NAL is a class I aldolase, and its biological role is to cleave Neu5Ac, however, at favorable conditions, the reverse aldol condensation reaction can be utilized in vitro to synthesize Neu5Ac from pyruvate and ManNAc. In this paper, we describe the recombinant production, biochemical characterization and structure determination of a N-acetylneuraminate lyase from the psychrophilic bacterium A. salmonicida (AsNAL). Despite having less than about 25% sequence identity to the homologous structures of EcNAL, HiNAL, SaNAL and PmNAL, AsNAL shares similarity in the overall fold, being a TIM barrel consisting of a barrel of 7 parallel strands (the eighth strand is distorted) surrounded by 11 helices. Although the sequence identity between AsNAL and the other NALs is low, residues involved in catalysis and substrate binding are well conserved.

A crystallization condition, composed of 25% PEG 1.5 K and 20% glycerol, produced diamond shaped crystals. The crystals diffracted up to 1.65 Å and belong to the orthorhombic space group I222 with cell parameters of 67 x 86 x 118 Å3. The whole amino acid sequence from residue 1 to 297 could be traced in the electron density maps. Three of the His residues from the tag were also visible in the electron density maps. Electron density clearly larger than water molecules was interpreted as glycerol and ethylene glycol originating from the crystallization conditions. There is one molecule in the asymmetric unit, but the crystallographic symmetry generates the functional tetrameric quaternary structure. The active sites are pointing inwards toward the center of a donut shaped tetramer. The corresponding residue in AsNAL is Asn168. This residue points towards the substrate and is positioned closer to the substrate than what is the case for Thr167 from EcNAL, or for an in silico mutation to threonine for AsNAL. Our structure of AsNAL shows that Asn168 is able to form two hydrogen bonds with substrates as ManNAc, Neu5Ac and Neu5Gc.

> MKKLTGLIAAPHTPFDSSSNVNFEEIDKIAKHLINDGVKGIYVCGTTGEGIHCSVEERKAIAERWVSACNHKLDIIVHTGALSIVDTLELTRHADTLDILATSAIGPCFFKPGSVSDLVEYCATIAAAAPSKGFYYYHSGMSGVNLNMEEFLIQADKRIPNLSGLKFNSGDLYEYQRCLRACDGKFDVPFGVDEFLPGALAVGAKSAVGSTYNYAAPHFNSIIEAFNKGDHDAVFNKMTNVIELIRVLVEFGGVAAGKIAMELHDINAGDPRLPLMPLSAEQKLTVVEKMRAANFLKHHH>[2x]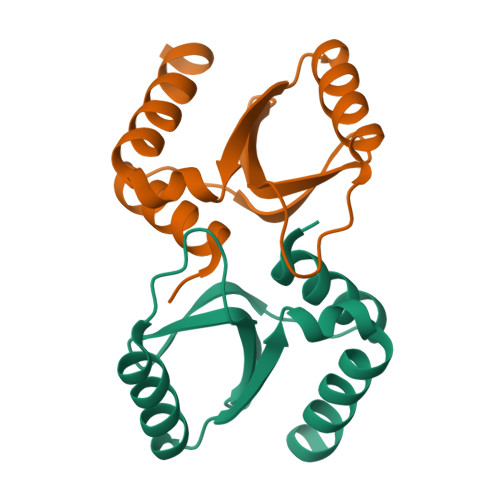GPLGSTTPERRVKEILDEMDIVYFTHHVVEGWNVAFYLGKKLAIEVNGVYWASKQKNVNKDKRKLSELHSKGYRVLTIEDDELNDIDKVKQQIQKFWVTHISNGM>MKVTLSALDTSESSFTPLVVIELAQDVKEETKEWLKNRIIAKKKDGGAQLLFRPLLNKYEQETLENQNLYLVGASKIRMLLGAEAVGLVKECNDNTMRAFTYRTRQNFKGFDDNNDDFLTMAECQFIIKHELENLRAKDEKMIPGYPQAKLYPGKSLLRRLLTSGIVIQVFPLHDSEALKKLEDTWYTRFALKYQPIDSIRGYFGETIALYFGFLEYFTFALIPMAVIGLPYYLFVWEDYDKYVIFASFNLIWSTVILELWKRGCANMTYRWGTLLMKRKFEEPRPGFHGVLGINSITGKEEPLYPSYKRQLRIYLVSLPFVCLC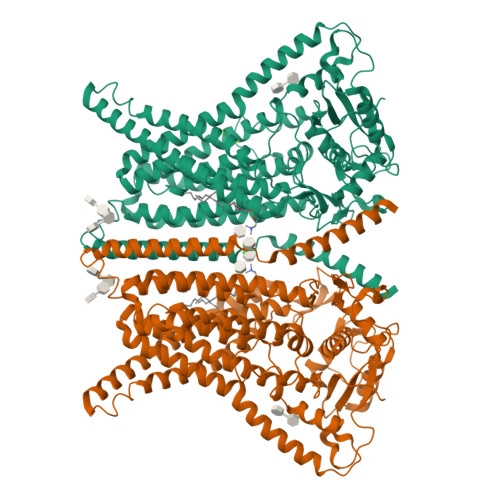LYFSLYVMMIYFDMEVWALGLHENSGSEWTSVLLYVPSIIYAIVIEIMNRLYRYAAEFLTSWENHRLESAYQNHLILKVLVFNFLNCFASLFYIAFVLKDMKLLRQSLATLLITSQILNQIMESFLPYWLQRKHGVRVKRKVQALKADIDATLYEQVILEKEMGTYLGTFDDYLELFLQFGYVSLFSCVYPLAAAFAVLNNFTEVNSDALKMCRVFKRPFSEPSANIGVWQLAFETMSVISVVTNCALIGMSPQVNAVFPESKADLILIVVAVEHALLALKFILAFAIPDKPRHIQMKLARLEFESLEALKQQQMKLVTENLKEEPMESGKEKATAENLYFQ[2x]6-chloro-N-{(3S)-1-[(2S)-1-{(1R,5S)-7-[2-(methylamino)ethyl]-3,7-diazabicyclo[3.3.1]non-3-yl}-1-oxopropan-2-yl]-2-oxopyrrolidin-3-yl}naphthalene-2-sulfonamide | C27 H36 Cl N5 O4 S | 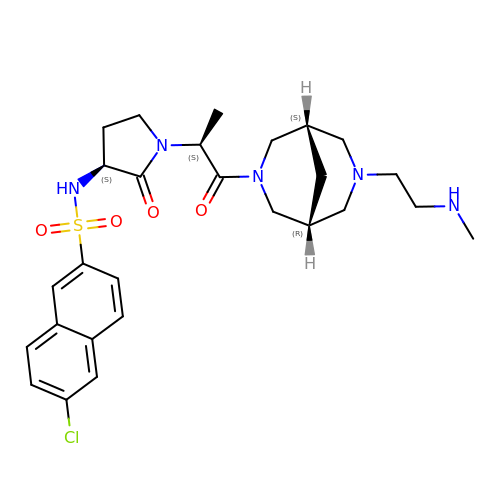NSTQUPKYMBYQSS-KSYXXAMZSA-N1-{1-[2-(hydroxymethyl)phenyl]-7-phenoxyindolizin-3-yl}ethanone 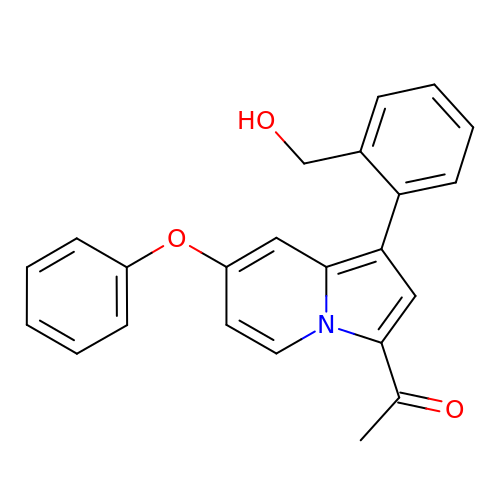| C23 H19 N O3 | AHWAKNWAECVAHU-UHFFFAOYSA-N When deamination affects guanosines, a xanthosine (X) containing RNA is generated. Applying NMR spectroscopy and X-ray crystallography, we demonstrate that X can form distinct wobble geometries with uridine depending on the sequence context. In contrast, X pairing with cytidine occurs either through wobble geometry involving protonated C or in Watson–Crick-like arrangement. We therefore utilized the 27 nt fragment of the E. coli 23S rRNA sarcin−ricin loop (SRL), the 12 nt RNA 5′-CGCGAAUUACGC, and the 14 nt RNA 5′-GGUAUUGCGGUACC, all of them are known crystallization scaffolds.

To maximize our chances to achieve a crystal structure also for the X–C base pair we tested a further RNA scaffold, namely 5′-GGUAUUGCGGUACC. Replacement of G10 and U5 by X10 and C5 indeed gave crystals that diffracted at 1.2 Å resolution. The structure of the self-complementary RNA shows a fully base-paired duplex with overall C2 symmetry, but strikingly, the two individual C–X pairs adopt distinct conformations. While C5′-X10 forms a wobble base pair, C5-X10′ forms a tridendate base pair that is equivalent in shape to a canonical G–C Watson Crick pair. The C5′–X10 wobble base pair is shape complementary to a typical G–U wooble pair (w1C–X in Figure 2D, F). Further, two ordered water molecules are observed, one bridging the the O2 of X10 and the 2′-OH of C5′ in the minor groove while the other one links the O6 of X10 and the C4-NH2 of C5′. Of note, for both X–C pairs, the riboses are all in C3′-endo conformation. With respect to the Watson–Crick shaped C5–X10′ pair, a tautomeric form of xanthosine must be involved, however, at the current state we are not able to distinguish between two interaction possibilities involving neutral nucleobases (top) versus charged nucleobases (bottom). Strikingly, we identified the two distinct X–C pairing modes in the X-ray structure of a palindromic RNA duplex, breaking C2 symmetry. This indicates that the two pairing modes are of comparable stability separated by low energetic barriers.

> GGUAXUGCGGUACC;> GGUACUGCGXUACC N-{4-METHYL-3-[(3-PYRIMIDIN-4-YLPYRIDIN-2-YL)AMINO]PHENYL}-3-(TRIFLUOROMETHYL)BENZAMIDE 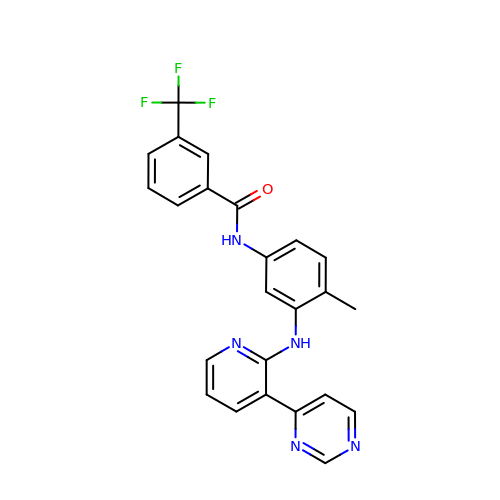| C24 H18 F3 N5 O | NESXBRNDMQUVNG-UHFFFAOYSA-N> SMKYKLNVLLAEIALIGTGNHY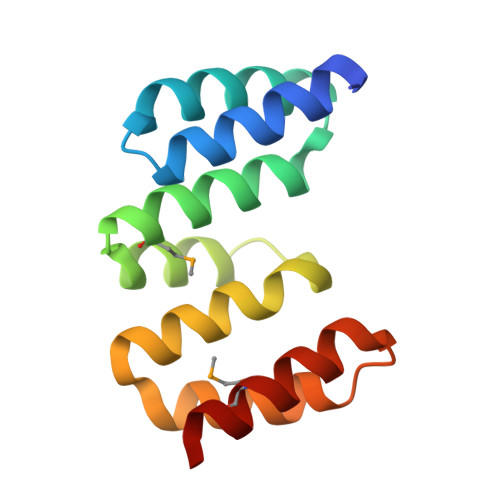HEEANCIAEWLHLKGEEEAVQLIRLSSLMNRGDYASALQQGNKLAYPDLEPWLALCEYRLGLGSALESRLNRLARSQDPRIQTFVNGMREQLKT> ALKPCEFPQFKYGRLYYEESLRPNFPVSIGNKYSYKCDNGFSP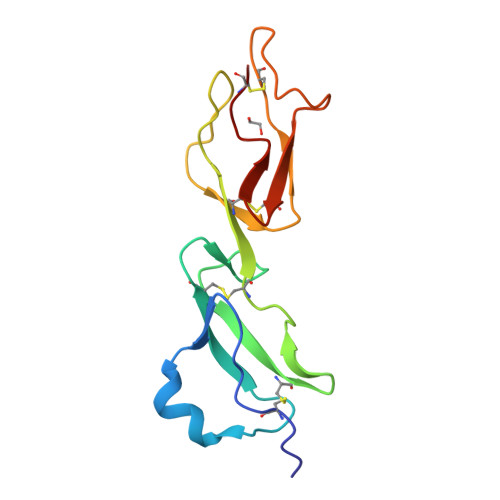PSGYSWDYLRCTAQGWEPEVPCVRKCVFHYVENGDSAYWEKVYVQGQSLKVQCYNGYSLQNGQDTMTCTENGWSPPPKCIR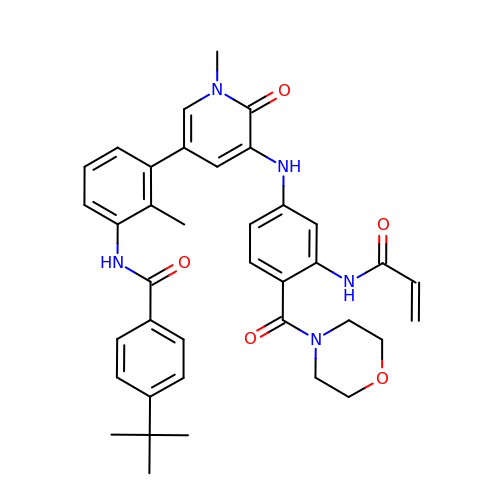N-[3-(5-{[3-(acryloylamino)-4-(morpholine-4-carbonyl)phenyl]amino}-1-methyl-6-oxo-1,6-dihydropyridin-3-yl)-2-methylphenyl]-4-tert-butylbenzamide | C38 H41 N5 O5 | UBXBHXGYYBYXOB-UHFFFAOYSA-N> MGLKLDLTWFDKSTEDFKGEEYSKDFGDDGSVMESLGVPFKDNVNNGCFDVIAEWVPLLQPYFNHQIDISDNEYFVSFDYRD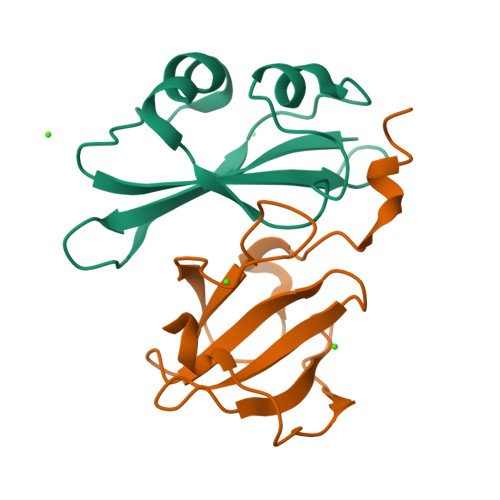GDW;> GFKDYGHDYHPAPKTENIKGLGDLKPGIPKTPKQNGGGKRKRWTGDKGRKIAEWDSQHGELEGYRASDGQHLGSFDPKTGNQLKGPDPKRNIKKYL> SGSAGNGLVPSDPVLAETMKNERVVQDHNSALRGARPINFGYLIKDAELKLVQSIKGSLRGSKLPPGHKGAHGRVSKTNGS;> SMANTIKVEGYPSMEWPTSLDIPLKASEELVGIDLETDLPDDPTDLKTLLVEESSEKEHWLTIALAYCNHGKTNEGIRLIEMALDVFQNSERASLHTFLTWAHLNLAKGHSLSVETKEHELTQAELNLKDAIGFDPTWIGNMLATVELYYQRGHYDKALETSDLFVKSIHAEDHRSGRQSKPNCLFLLLRAKLLYQKKNYVASLKIFQELLVINPVLQPDPRIGIGLCFWQLKDPKMAIKSWQRALQINSKNTSASILVLLGEFHNSLTDSTNDEVFKETFSKALSDLKNIFSENQNNPVLLTLLQTYHYFKGDFQTVLDIYHHKILKMSPLIAKTVLSESSFWCGRAHYALGDYRKSFIMFQESLKKNEDNLMARLGLGQTQIKSNLLEESIITFENLYKTNESLQELNYILGLLYAGKTLDVKTSKSIPAKELNKLNEKALQYLERYIKLTVAKKNQLIISRVYLVISQLYESQNQYKISLDFLSKALEEMEFVNKDEVPLEILNNLACYHFINGDLTKADNLFEQAKAKVSDMNKSVNITLEYNIARTSEKTNWEKSESIYSQITSSHPSYISARIRNLYIKFAHSKINDSEMNIEINGLLEMNKSDLEMRSFYGWYLKNSEERKNSEKSTSHNKETLVKYNSHDAYALISLANLYVTIARDGKKSRNPKEQEKSKHSYLKAIQLYQKVLQIDPFNVFAAQGVAIIFAESKRLGPALEILRKIRDSLDNEDVQLNLAHCLLEMREFGKAIENYELVLKKFDNERTRPHILNLLGRAWYSRGMKERSVSFFQKALENAKTALELFVQQSAKNKFIHSVKFNIALLQFQIAETLRRSNPKFRTVQQIKDSLEGLEEGLALFKELNDLKEFNMIPKEELEQRIQLGETTMKSALERSLNEQEEFEKDQ;> SMSKKQEYIAPIKYQNSLPVPQLPPKLLAYPEAPETNPDSSQLINSLYVKTNISNLIQQDEDLGMPVDLMKFPGLLNKLDSKLLYGFDNVKLDKDDRILLRDPRIDRLTKT;> SKSDPFSRLKTRTKVYYQEIQKEENAKAKEMAQQEKLQEDRETKERREKELLLAQFRRLGGLERMIGELDIKFDFKF

The polymerase-associated factor 1 complex (PAF1C) is one of the most important transcription elongation factors that positively regulates genome-wide gene expression. In simple eukaryotes such as budding yeast, PAF1C contains five subunits: Paf1, Ctr9, Cdc73, Leo1 and Rtf1. PAF1C can regulate transcription through direct association with the polymerase or by impacting the chromatin structure epigenetically. The largest component, Ctr9, forms the backbone and shapes the overall architecture of the complex, while the other components join the complex mainly through associations with Ctr9.

We found that PAF1C from the yeast Saccharomyces eubayanus, which showed 86% sequence identity from that of budding yeast, could be purified and produce better crystals. We then optimized the crystals of the complex of Ctr9-Paf1-Cdc73-Rtf1 from Saccharomyces eubayanus and solved the structure at the resolution of 2.7 Å. The overall architecture of the Ctr9-Paf1-Cdc73-Rtf1 quaternary complex from Saccharomyces eubayanus was shown to be similar as to those from the thermophilic fungus and from humans. The major body of Ctr9 folds into 21 tetratricopeptide repeats (TPRs) that wrap around the N-terminus of Paf1 to form a three-circled right-handed solenoid structure, with the Paf1 N-terminus just filling in the central tunnel of the Ctr9 solenoid. To facilitate crystallization, the C-terminal long α helix was truncated. Paf1 residues 9–105 can be traced in the Ctr9-Paf1-Cdc73-Rtf1 quaternary complex. Cdc73 joins PAF1C mainly through its middle region, which contains two helices connected by loops, and contacts Ctr9 spanning a region containing the lower part of the middle turn and the upper part of the C-terminal turn. The overall structure of Rtf1 (residues 502 to 570) in the quaternary complex has the shape of a twisted letter “U” that contains three α helices connected by loops. In our study, we observed that helix α1 of Rtf1 actually interacts with a new surface made of Ctr9 and Paf1. With this additional binding surface, the total contact surfaces between Rtf1 and the PAF1C core subunits from Saccharomyces eubayanus reached to 3025 Å2, which is much larger than the corresponding contact surfaces from Saccharomyces cerevisiae or Komagataella phaffii, which are 1754 Å2 or 1509 Å2, respectively.Endoplasmic reticulum (ER) membrane resident P5A-ATPases broadly affect protein biogenesis and quality control, and yet their molecular function remains debated. Here, we report cryo-EM structures of a P5A-ATPase, CtSpf1, covering multiple transport intermediates of the E1 → E1-ATP → E1P-ADP → E1P → E2P → E2.Pi → E2 → E1 cycle. All P-type ATPases share a common fold with a transmembrane (M) domain responsible for cargo transport across the membranes, and actuator (A), nucleotide binding (N), and phosphorylation (P) domains handling ATP turnover. Collectively, our findings are compatible with a broad range of proteins as cargo, with the P5A-ATPases serving a role in membrane removal of helices, although insertion/secretion cannot be excluded, as well as with a mechanistic role of the Plug-domain.

Subsequently, we also recovered an apo CtSpf1 structure, isolated without the presence of state-stabilizing agents or inhibitors, determined at an overall resolution of 3.4 Å with well-resolved domains. Structure-based alignments of the structure to P2-, P4-, and P5-ATPases indicate it resembles an E1 or E1-ATP state, which is typically associated with “inward-open” or “inward-facing occluded” configurations, respectively (RMSD 5.5, 5.0, 5.7, 2.2, and 3.0 Å to PDB-IDs 4H1W56, 3N8G57, 6K7G58, 6XMP23, and 7N7513, respectively). In the M-domain, we find a deep cytosol-facing crevice, in-between primarily M2, M4, and M6 but partially lined also by M1 and M8, that deviates substantially from the cleft identified in the E2P/E2.Pi states. The cavity, together with the arrangement of the soluble domains, renders us denoting the state E1. The identified inward-open crevice likely represents a critical aspect of the transport pathway, since the opening is overlaying the cleft of the M-domain in the E2P/E2.Pi states, and the cleft is lined by E458 and E462. However, the cavity is blocked by the C-terminal portion of the P-domain insertion, with residues 1005–1013 dipping into the membrane and inserting between M2 and M4, hence forming another link between the soluble and M-domains. Moreover, the apo cryo-EM data yielded two maps of the same resolution, where the only difference is the relative position of the P-domain insertion relative to the ATPase core, revealing additional flexibility. The observed ability of this P-domain insertion to block the likely transport pathway in the M-domain lead us to rename it the Plug-domain and the C-terminal residues of the domain (residues 1005–1013 model, but non-sharpened maps suggest it extends beyond D1005) the Plug, the significance of which will be discussed later. P5A-ATPases seemingly rest in a cytosol-facing E1 state, which is blocked by the Plug domain (green). The closing of the ER luminal end of the cleft would then push the helix into the cytoplasm, and following release, the cytoplasmic cavity is capped by the Plug-domain, as observed in our E1 structure.

> MAPLVDNPQIKSAELLRPLPLYQHAYVWPYVIVWPVFLRVYLTQELYDKYIGAQEWTFVWIISIVTFQTLTWLCTHWSVNLNALFTAKKASSIEDAQLIKVIPVANAGAADICKLVRDKVGDNKTNISFLFQKRRFLWYPERKAFSTLEFDIDAEPKPTLSKFQLSRGIESEDELKRLEQHYGTNTFDIPVPTFTELFKEHAVAPFFVFQVFCVGLWLLDEYWYYSLFTLVMLVVFESTVVWQRQRTLTEFRSMSIKPYPIYVYRLGKWTEIQSDKLLPGDLVSVTRTKEDSGVACDMILVEGTAIVNEAMLSGESTPLLKDSIQLRPGDAVLEVDGLDKNSLLWGGTKVLQITHGTAEEERPKPASGIPPPPDNGAMAVVTKTGFETSQGSLVRTMIYSTERVSANNTEALLFILFLLVFALAASWYVWDEGVRKDRKRSKLLLDCILIITSVVPPELPMELSLAVNTSLSALAKFAIFCTEPFRIPFAGRIDVACFDKTGTLTGEDLVVEGIAGLGLGHSGTDTPKEADGAHTRMVSVHDAGMETTLVLATAHALVKLDEGEIVGDPMEKATLNALGWVLGKNDTLTSKPGNAASSGILGTVQIKRRFQFSSALKRQSSVATITATEVKTGRKLRGSFVGVKGAPETIMKMLVTVPEHYEETYKYFTRRGSRVLALAYKQLTTEGELGANKINDLKRESVEADLHFAGFLVLQCPLKEDAKQAVRMLNESSHRVVMITGDNPLTAVHVAKEVEIVDRDVLILDAPEHSVYGEESLVWRSVDDKIRIDVDPTKPIDPEILKTKDLCVTGYALNKFKGQVGWKSLLRYTWVYARVSPKQKEDILLGLKDMGYYTLMAGDGTNDVGALKQAHVGVALLNGTQEDLNRIAEHTRNQKMKELYQKQVDLMARWGQPPPPVPAMIAHLYPPGPSNPHYQKAMEREAQKRGVTVEQLAKVNGTNVTSNPAGVQQQSGQDAKKAKQVEAAKKAANFADKLTSSLMEAEMDDEPPTLKLGDASVAAPFTSKLRNVMAIPNILRQGRCTLVATIQMYKILALNCLISAYSLSVLYLEGIKFGDGQITISGMLMSVCFLSISRARSVEGLSKERPQPNIFNFYIIGSILGQFAVHVATLIYIAQLCDQIEPRTEVIDLEAEFKPSLLNSAVYLLQLIQQISTFAVNYQGRPFRESLSENKGMFYGIVGVTAIAFACSTEMLPELNEAMKLVPFNENFKTIMTTVMIIDFVACYVIEWVLKKLFSDLRARDIAERRPDQLERERVRKEKEAREKEEEEERKERERIEAFERRLEEKRTRLVEAAAQREQQQQQWAQRR>[10x]MQEVQSSRSGRGGNFGFGDSRGGGGNFGPGPGSNFRGGSDGYGSGRGFGDGYNGYGGGPGGGNFGGSPGYGGGRGGYGGGGPGYGNQGGGYGGGYDNYGGGNYGSGNYNVFGNYNQQPSNY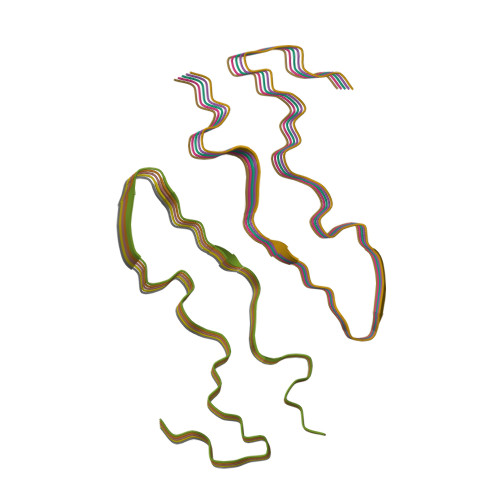GPMKSGNFGGSRNMGGPYGGGNYGPGGSGGSGGYGGRSRY> MPVAGSELPRRPLPPAAQERDAEPRPPHGELQYLGQIQHILRCGV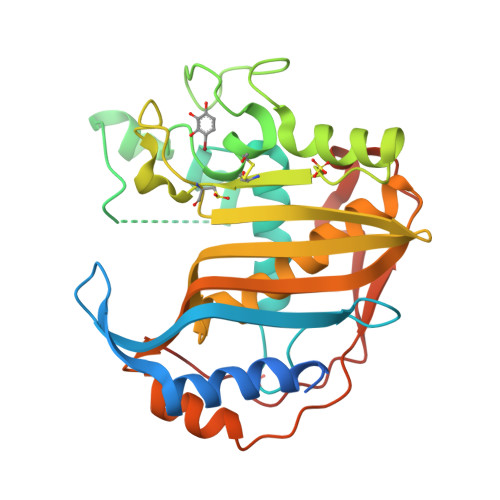RKDDRTGTGTLSVFGMQARYSLRDEFPLLTTKRVFWKGVLEELLWFIKGSTNAKELSSKGVKIWDANGSRDFLDSLGFSTREEGDLGPVYGFQWRHFGAEYRDMESDYSGQGVDQLQRVIDTIKTNPDDRRIIMCAWNPRDLPLKALPPCHALCQFYVVNSELSCQLYQRSGDMGLGVPFNIASYALLTYMIAHITGLKPGDFIHTLGDAHIYLNHIEPLKIQLQREPRPFPKLRILRKVEKIDDFKAEDFQIEGYNPHPTIKMEMAV2-chloro-4-({5-[(2,6-difluorophenyl)methyl]-1,3-oxazol-2-yl}amino)benzonitrile | C17 H10 Cl F2 N3 O | 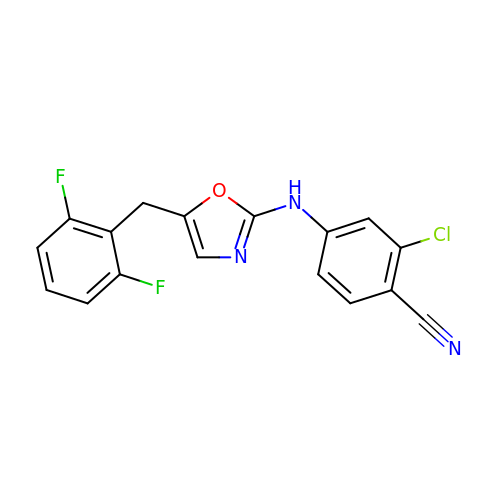XMNGPECGUKASMW-UHFFFAOYSA-N Type 4 pili (T4P) are retractable surface appendages found on numerous bacteria and archaea that play essential roles in various microbial functions, including host colonization by pathogens. T4P are composed of thousands of copies of a major pilin protein arranged in a helical array. They are assembled and retracted by a complex machine composed of several essential proteins, including a dedicated extension ATPase, most often called PilB, that is essential for pilus biogenesis. Here, we report the cryo-electron microscopy (cryo-EM) structure of the BfpD ATPase from enteropathogenic Escherichia coli (EPEC) in the presence of either ADP or a mixture of ADP and AMP-PNP. Both structures, solved at 3 Å resolution, reveal the typical toroid shape of AAA+ ATPases and unambiguous 6-fold symmetry.

Purified BfpD was prepared under two nucleotide conditions: either in the presence of ADP (BfpD-ADP data set) or in the presence of ADP, ATP, and the nonhydrolysable ATP analog, AMP-PNP (termed BfpD-ANP data set) at a ratio of 2:4:5. For BfpD-ANP, a data set of 9,853 good movies and 424,708 good particles with well-distributed orientation yielded two classes, with 214,673 and 58,944 particles, respectively. Subsequent 3D reconstruction with C6 symmetry yielded resolutions of 3.1 Å, 3.0 Å, and 3.7 Å for BfpD-ADP, BfpD-ANP class-1 and BfpD-ANP class-2, respectively. For the BfpD-ANP data set, despite the addition of ADP, ATP, and AMP-PNP, the active site of all monomers was fully occupied by electron density consistent with AMP-PNP, suggesting that ultimately ANP occupied the active sites and remained there. The presence of ANP in the catalytic site results in an outward N2D movement, stabilized by interaction between Arg 217 and the γ-phosphate. BfpD-ANP class-1 has an outward N2D compared to BfpD-ANP class-2. Comparison of the BfpD-ADP and BfpD-ANP structures reveals a subtle outward shift in position of the N2D with respect to the CTD such that the mobile innermost N2D loops delineate a circle of 65 Å in diameter (distance between diagonally located Ala172 residues) in the presence of ADP, and 70–73 Å diameter in the presence of ANP class 1 and 2, respectively. The N2D moves toward the 6-fold axis in going from ANP class-2 to ANP-class-1, likely reflecting two successive steps on the way to ATP hydrolysis. The ring contraction from class-2 to class-1 is accompanied by loss of contact between the ATP-stabilizing Arg217 and the Ɣ phosphate of ATP, and gradual shortening of the distance between the catalytic residue Glu295 and that same phosphate, priming the active site for catalysis. As Glu338 and the catalytic glutamate Glu295 are 5.3–11.6 Å away from the γ-phosphate of ANP, it appears that the ATPase captured by cryo-EM is a prehydrolysis intermediate between the ADP/ATP exchange and ATP hydrolysis steps of the catalysis cycle.

>[6x]MVNKTEKTSDLMFERFKRNVSEIVTGDGGELELTVEQRKYFLIFKNGDFLVSSCHMKHHLVQMLREIATRKGYPNLTIYEVNLKDIRLLYEASLKTVQNNGQDLLPVEKRASMLLFECAEMRVSDLHIKVYDAEADIYIRKDGDMELLRQIESNTAHSILASLYNNADDSDATYKINAYQAARIVASKSRLALPPVIQAVRLQFNPLGQGGRYLIARFLYTDKSEKQKEMDPTRFGFHHSHAESFSRMRNLPIGINIISGPTGSGKSTTLKNLLELLYIEKKKKVNIISIEDPPEYEIDGTAQLPITNVETEAQRGEEYRKAITAALRSDPDIIMPGEARDAEVINLLFTAAMTGHQVWTSLHANNALAIFDRLKDQGVDEFKLTDPELITGLVAQRLVRKLCAQCSITLTEYIASGGGISDTDRKIISGHETSVRFPNPRAKKCCRDGYNGRTILAEVIEPDSKLLRLVAEGKREDAQHYWLTSLHGMALKEHAWLKIISGEICVMDAVNKISGIDNITEERKKYLFSRDNEI> MDCRNLCGAAAPSRLVQPGCFICRGVAVSIPPAAPGPATSVFDTPPSTFSLRPDGTIIAGTGIRGDHASVGTDGTIEMFIVPFIGDVTGSELTHPYAVELQDGEELAIAFGVTLKSGYGARITEYYDVSLFLENGGNSKELTLQPANTKSGYVWSDGHGYNITDSDGDLHTVQNVTRPVWFEM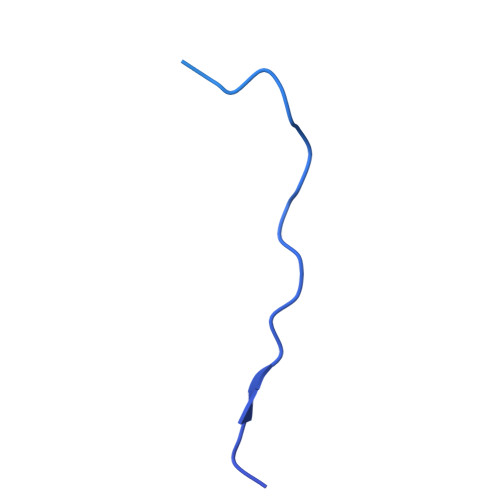TEPGIVGVIMEARYKATGLVSSSISITVNVTYAD>[2x]GAGEARLEEAVNRWVLKFYFHEALRAFRGSRYGDFRQIRDIMQALLVRPLGKEHTVSRLLRVMQCLSRIEEGENLDCSFDMEAELTPLESAINVLEMIKTEFTLTEAVVESSRKLVKEAAVIICIKNKEFEKASKILKKHMSKDPTTQKLRNDLLNIIREKNLAHPVIQNFSYETFQQKMLRFLESHLDDAEPYLLTMAKKALKSESAASST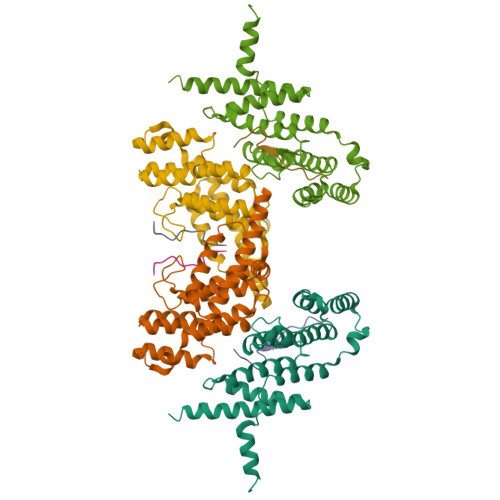GKEDKQPAPGPVEKPPREPARQL;>SFNLAPLGRRRVQSQWAST[2x]>SNALQHTTIGDVLREHRRSHPGRTALVDGPVRLTWPELDDRVNRLAGSLAASGIGRGDRIMWLGQNSFRVYELIAAAGKLGAMVCVGYWRWAPPEMEFALRDFDPHLVVWQHQEIHETVARTREALGSDDTARWLRHDSAPQDPDGYEAFLAAGGLADPDLDIDPDSPVLVLYTAAMSGRQCGSLLSHTNLIAMATAAAWLGDIDHTTAFLNSGPMFHIGNHQFWGMPTLLMAGKNVIVRRVVAEEVRDLLVAEECTHAFLMPPTVAEIVRLNRDTGHDLSRLRATVAPHLWEGMATTDTSRFTRSGAAAGRGY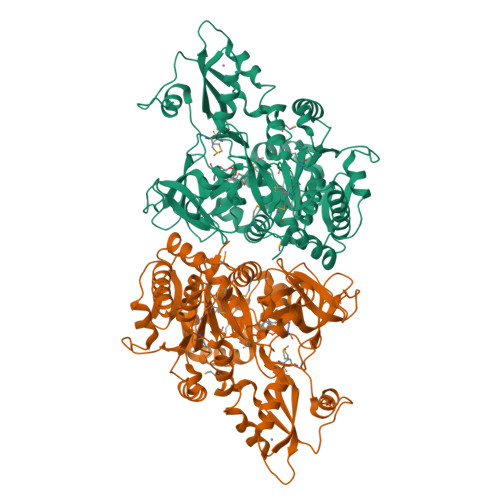GQTELSGFAVTAAYGGPAAGNAGRPGPGLTVRVLDTAGRECAVGEAGEICARGTVVHRGYWNRDEVNAHRFRSGWWHTTDLGRREPDGSLTFLGTTTRMLKSAAENIFPAEVENCIEQHPAVREAAVIGVPNTRWAQDVKAVVVLEPDAGVSEQEIIDHCRPRIASYKKPKSVAFAAALPRTVSGARDYDALDKEYGGGGYPGAATLGPGR[2x]> MQIPRDVIFEVVRGFRGRSRNCIKIARVRAMKALLYSYIMRRQ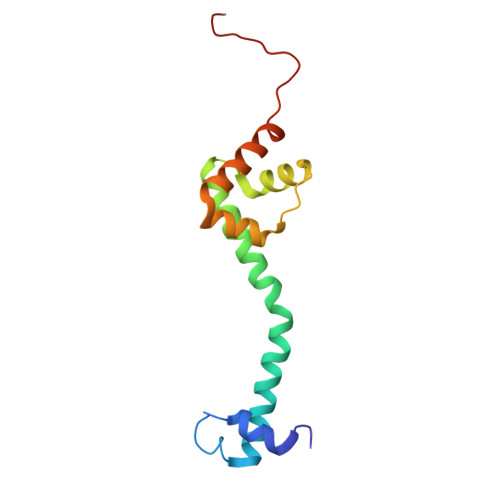RQRRYRVFWIGRINAAGREWSFPYAWLATSLWRQNIWLDRKMLANLAETEPASFRALVNEGKSVYFWNPDKVRDIQDL> EEQWAREIGAQ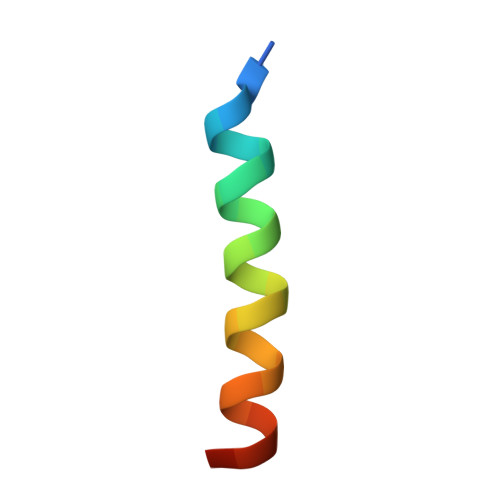LRRMADDLNAQYER> MRRETVGEFSSDDDDDILLELGTRPPRFTQIPPSSAALQTQIPTTLEVTTTTLNNKQSKND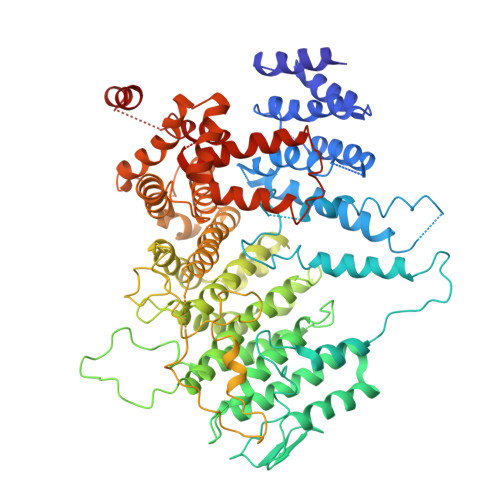NQLVNQLNKAQGEASMLRDKINFLNIEREKEKNIQAVKVNELQVKHLQELAKLKQELQKLEDEKKFLQMEARGKSKREVITNVKPPSTTLSTNTNTITPDSSSVAIEAKPQSPQSKKRKISDNLLKKNMVPLNPNRIIPDETSLFLESILLHQIIGADLSTIEILNRLKLDYITEFKFKNFVIAKGAPIGKSIVSLLLRCKKTLTLDRFIDTLLEDIAVLIKEISVHPNESKLAVPFLVALMYQIVQFRPSATHNLALKDCFLFICDLIRIYHHVLKVPIHESNMNLHVEPQIFQYELIDYLIISYSFDLLEGILRVLQSHPKQTYMEFFDENILKSFEFVYKLALTISYKPMVNVIFSAVEVVNIITSIILNMDNSSDLKSLISGSWWRDCITRLYALLEKEIKSGDVYNENVDTTTLHMSKYHDFFGLIRNIGDNELGGLISKLIYTDRLQSVPRVISKEDIGMDSDKFTAPIIGYKMEKWLLKLKDEVLNIFENLLMIYGDDATIVNGEMLIHSSKFLSREQALMIERYVGQDSPNLDLRCHLIEHTLTIIYRLWKDHFKQLREEQIKQVESQLIMSLWRFLVCQTETVTANEREMRDHRHLVDSLHDLTIKDQASYYEDAFEDLPEYIEEELKMQLNKRTGRIMQVKYDEKFQEMARTILESKSFDLTTLEEADSLYISMGL>MTTEQRRSLQAFQDYIRKTLDPTYILSYMAPWFREEEVQYIQAEKNNKGPMEAATLFLKFLLELQEEGWFRGFLDALDHAGYSGLYEAIESWDFKKIEKLEEYRLLLKRLQPEFKTRIIPTDIISDLSECLINQECEEILQICSTKGMMAGAEKLVECLLRSDKENWPKTLKLALEKERNKFSELWIVEKGIKDVETEDLEDKMETSDIQIFYQEDPECQNLSENSCPPSEVSDTNLYSPFKPRNYQLELALPAMKGKNTIICAPTGCGKTFVSLLICEHHLKKFPQGQKGKVVFFANQIPVYEQQKSVFSKYFERHGYRVTGISGATAENVPVEQIVENNDIIILTPQILVNNLKKGTIPSLSIFTLMIFDECHNTSKQHPYNMIMFNYLDQKLGGSSGPLPQVIGLTASVGVGDAKNTDEALDYICKLCASLDASVIATVKHNLEELEQVVYKPQKFFRKVESRISDKFKYIIAQLMRDTESLAKRICKDLENLSQIQNREFGTQKYEQWIVTVQKACMVFQMPDKDEESRICKALFLYTSHLRKYNDALIISEHARMKDALDYLKDFFSNVRAAGFDEIEQDLTQRFEEKLQELESVSRDPSNENPKLEDLCFILQEEYHLNPETITILFVKTRALVDALKNWIEGNPKLSFLKPGILTGRGKTNQNTGMTLPAQKCILDAFKASGDHNILIATSVADEGIDIAQCNLVILYEYVGNVIKMIQTRGRGRARGSKCFLLTSNAGVIEKEQINMYKEKMMNDSILRLQTWDEAVFREKILHIQTHEKFIRDSQEKPKPVPDKENKKLLCRKCKALACYTADVRVIEECHYTVLGDAFKECFVSRPHPKPKQFSSFEKRAKIFCARQNCSHDWGIHVKYKTFEIPVIKIESFVVEDIATGVQTLYSKWKDFHFEKIPFDPAEMSK[2x];>MAGLGLGSAVPVWLAEDDLGCIICQGLLDWPATLPCGHSFCRHCLEALWGARDARRWACPTCRQGAAQQPHLRKNTLLQDLADKYRRAAREIQAGSDPAHCPCPGSSSLSSAAARPRRRPELQRVAVEKSITEVAQELTELVEHLVDIVRSLQNQRPLSESGPDNELSILGKAFSSGVDLSMASPKLVTSDTAAGKIRDILHDLEEIQEKLQESVTWKEAPEAQMQGELLEAPSSSSCPLPDQSHPALRRASRFAQWAIHPTFNLKSLSCSLEVSKDSRTVTVSHRPQPYRWSCERFSTSQVLCSQALSSGKHYWEVDTRNCSHWAVGVASWEMSRDQVLGRTMDSCCVEWKGTSQLSAWHMVKETVLGSDRPGVVGIWLNLEEGKLAFYSVDNQEKLLYECTISASSPLYPAFWLYGLHPGNYLIIKQVKV[2x]

RIG-I is an essential innate immune receptor that responds to infection by RNA viruses. The RIG-I signaling cascade is mediated by a series of post-translational modifications, the most important of which is ubiquitination of the RIG-I Caspase Recruitment Domains (CARDs) by E3 ligase Riplet. Riplet is a homodimer composed of an N-terminal RING domain (catalytic domain), CC domain (coiled-coil domain, homodimerization), and C-terminal PrySpry domain (RIG-I recognition domain). Each structure contains two RIG-I molecules, one p3dsRNA24, and one Riplet homodimer, but they differ in the relative positions of two PrySpry domains, which depend on the relative positions of their partner RIG-I molecules.

Given that the footprint of RIG-I on dsRNA is ~10 bp, we designed a 24-basepaired dsRNA (p3dsRNA24) bearing two 5′-triphosphorylated blunt dsRNA termini for recruiting two RIG-I molecules. Indeed, p3dsRNA24 successfully forms a stable ternary complex, resulting in a significantly enhanced Riplet KD (from 700 nM to 6.6 nM), enabling large-scale purification of the complex for subsequent structural work. In the structure reconstructed from the major population of particles (70.1%), each triphosphorylated terminus is bound to an individual RIG-I molecule (end-bound complex), thereby enabling the Riplet proteins to adopt a head-to-head arrangement. In this case, each PrySpry domain recognizes a specific motif on the outer surface of RIG-I Hel2. Despite the different relative orientations of PrySpry in the three structures, the PrySpry domain uses the same interface with RIG-I Hel2 in each case. Using the major particle class as an example, the interacting interface buries a comparatively small solvent-accessible surface area (889.5 Å2 on average, 1200–1700 Å2 for antigen-antibody complex), consistent with the low affinity between Riplet and apo-RIG-I/RIG-I:p3SLR14 (0.7 µM). At this interface, the Riplet PrySpry domain uses several loops to recognize a rigid motif composed of an α-helix in the outer surface of the RIG-I Hel2 domain. The side chains of W415, Y417, and L419 in PrySpry insert into the hydrophobic pockets formed by F616, I617 and L624, while R342 and E350 in PrySpry make polar contacts with RIG-I Hel2, resulting in an interface that is consistent with the first RIG-I:Riplet structures obtained using artificially fused RipletPrySpry-RIG-IΔCARDs 23. Single point mutations in Riplet, including F616A, I617A, and L624A in RIG-I and W415A, Y417A, and L419D, which are located at the RIG-I:Riplet interface, drastically diminished the IFN response in the context of RNA ligand p3SLR14. This finding confirms that Riplet interacts with RIG-I:p3SLR14 under physiological conditions in the same way as that illustrated by the structural work using p3dsRNA24.>APPSVFAEVPQAQPVLVFKLIADFREDPDPRKVNLGVGAYRTDDCQPWVLPVVRKVEQRIANNSSLNHEYLPILGLAEFRTCASRLALGDDSPALQEKRVGGVQSLGGTGALRIGAEFLARWYNGTNNKDTPVYVSSPTWENHNGVFTTAGFKDIRSYRYWDTEKRGLDLQGFLSDLENAPEFSIFVLHACAHNPTGTDPTPEQWKQIASVMKRRFLFPFFDSAYQGFASGNLEKDAWAIRYFVSEGFELFCAQSFSKNFGLYNERVGNLTVVAKEPDSILRVLSQMQKIVRVTWSNPPAQGARIVARTLSDPELFHEWTGNVKTMADRILSMRSELRARLEALKTPGTWNHITDQIGMFSFTGLNP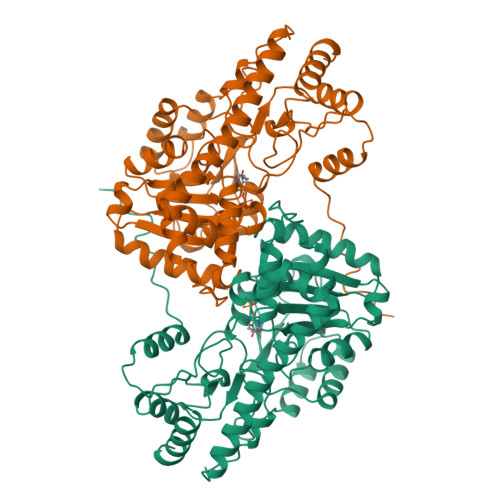KQVEYLINQKHIYLLPSGRINMCGLTTKNLDYVATSIHEAVTKIQ[2x]> MTTELNQGEQFVADFRANAAALTTANAYNPEDEHDACGVGFIAAIDGKPRRSVVEKGIEALKAVWHRGAVDADGKTGDGAGIHVAVPQKFFKDHVKVIGHRAPDNKLAVGQVFLPRISLDAQEACRCIVETEILAFGYYIYGWRQVPINVDIIGEKANATRPEIEQIIVGNNKGVSDEQFELDLYIIRRRIEKAVKGEQINDFYICSLSARSIIYKGMFLAEQLTTFYPDLLDERFESDFAIYHQRYSTNTFPTWPLAQPFRMLAHNGEINTVKGNVNWMKAHETRMEHPAFGTHMQDLKPVIGVGLSDSGSLDTVFEVMVRAGRTAPMVKMMLVPQALTSSQTTPDNHKALIQYCNSVMEPWDGPAALAMTDGRWVVGGMDRNGLRPMRYTITTDGLIIGGSETGMVKIDETQVIEKGRLGPGEMIAVDLQSGKLYRDRELKDHLATLKPWDKWVQNTTHLDELVKTASLKGEPSDMDKAELRRRQQAFGLTMEDMELILHPMVEDGKEAIGSMGDDSPIAVLSDKYRGLHHFFRQNFSQVTNPPIDSLRERRVMSLKTRLGNLGNILDEDETQTRLLQLESPVLTTAEFRAMRDYMGDTAAEIDATFPVDGGPEALRDALRRIRQ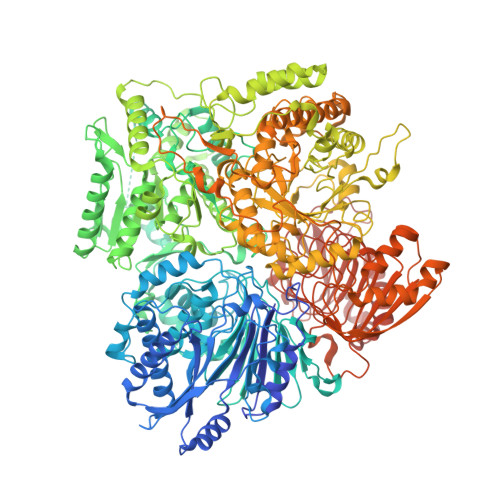ETEDAVRGGATHVILTDEAMGPARAAIPAILATGAVHTHLIRSNLRTFTSLNVRTAEGLDTHYFAVLIGVGATTVNAYLAQEAIAERHRRGLFGSMPLEKGMANYKKAIDDGLLKIMSKMGISVISSYRGGGNFEAIGLSRALVAEHFPAMVSRISGIGLNGIQKKVLEQHATAYNEEVVALPVGGFYRFRKSGDRHGWEGGVIHTLQQAVTNDSYTTFKKYSEQVNKRPPMQLRDLLELRSTKAPVPVDEVESITAIRKRFITPGMSMGALSPEAHGTLNVAMNRIGAKSDSGEGGEDPARFRPDKNGDNWNSAIKQVASGRFGVTAEYLNQCRELEIKVAQGAKPGEGGQLPGFKVTEMIARLRHSTPGVMLISPPPHHDIYSIEDLAQLIYDLKQINPDAKVTVKLVSRSGIGTIAAGVAKANADIILISGNSGGTGASPQTSIKFAGLPWEMGLSEVHQVLTLNRLRHRVRLRTDGGLKTGRDIVIAAMLGAEEFGIGTASLIAMGCIMVRQCHSNTCPVGVCVQDDKLRQKFVGTPEKVVNLFTFLAEEVREILAGLGFRSLNEVIGRTDLLHQVSRGAEHLDDLDLNPRLAQVDPGENARYCTLQGRNEVPDTLDARIVADARPLFEEGEKMQLAYNARNTQRAIGTRLSSMVTRKFGMFGLQPGHITIRLRGTAGQSLGAFAVQGIKLEVMGDANDYVGKGLSGGTIVVRPTTSSPLETNKNTIIGNTVLYGATAGKLFAAGQAGERFAVRNSGATVVVEGCGSNGCEYMTGGTAVILGRVGDNFAAGMTGGMAYVYDLDDSLPLYINDESVIFQRIEVGHYESQLKHLIEEHVTETQSRFAAEILNDWAREVTKFWQVVPKEMLNRLEVPVHLPKAISAE>[3x]LRIPNIATYTGTIQGKGEVCIIGNKEGKTRGGELYAVLHSTNVN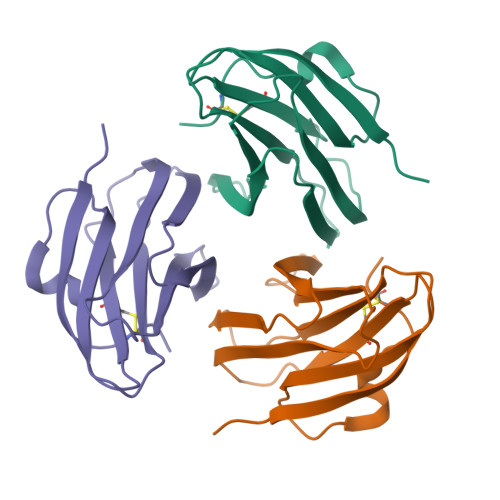ADMTLILLRNVGGNGWGEIKRNDIDKPLKYEDYYTSGLSWIWKIKNNSSETSNYSLDATVHDDKEDSDVLTKCPV>SEFELRSRYFIMLCDNETAIAHAKKTSIWAVKKDSSKRISDAYKKASVYFIFVAQQTYNALGYAQVVSDLNSTELPFWSDSSHAGGVRIKWIKTCN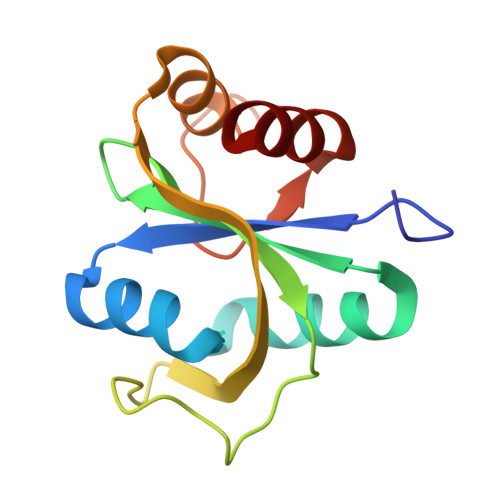LFSAEISEIVSHMDHGSEARDGMEMMYDEGSRLCTLIN[2x]(3R)-1-{4-[{4-chloro-2-[(S)-(2-chlorophenyl)(hydroxy)methyl]phenyl}(2,2-dimethylpropyl)amino]-4-oxobutanoyl}piperidine-3-carboxylic 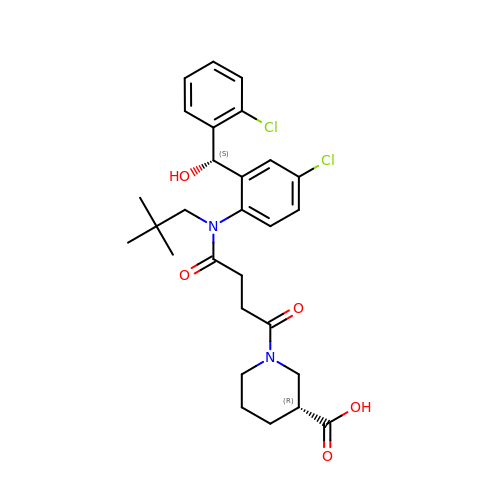acid | C28 H34 Cl2 N2 O5 | SGSZXPGOMQXFLD-WXTAPIANSA-N> APLVHHHHHHALDENLYFQGALAKYAPDENCPDQNPRLRNWDPGQDSAKQVVIKEGDMLRLTSDATVHSIVIQDGGLLVFGDNKDGSRNITLRTHYILIQDGGALHIGAEKCRYKSKATITLYGKSDEGESMPTFGKKFIGVEAGGTLELHGARKASWTLLARTLNSSGLPFGSYTFEKDFSRGLNVRVIDQDTAKILESERFDTHEYRNESRRLQEFLRFQDPGRIVAIAVGDSAAKSLLQGTIQMIQERLGSELIQGLGYRQAWALVGVIDGGSTSCNESVRNYENHSSGGKALAQREFYTVDGQKFSVTAYSEWIEGVSLSGFRVEVVDGVKLNLLDDVSSWKPGDQIVVASTDYSMYQAEEFTLLPCSECSHFQVKVKETPQFLHMGEIIDGVDMRAEVGILTRNIVIQGEVEDSCYAENQCQFFDYDTFGGHIMIMKNFTSVHLSYVELKHMGQQQMGRYPVHFHLCGDVDYKGGYRHATFVDGLSIHHSFSRCITVHGTNGLLIKDTIGFDTLGHCFFLEDGIEQRNTLFHNLGLLTKPGTLLPTDRNNSMCTTMRDKVFGNYIPVPATDCMAVSTFWIAHPNNNLINNAAAGSQDAGIWYLFHKEPTGESSGLQLLAKPELTPLGIFYNNRVHSNFKAGLFIDKGVKTTNSSAADPREYLCLDNSARFRPHQDANPEKPRVAALIDRLIAFKNNDNGAWVRGGDIIVQNSAFADNGIGLTFASDGSFPSDEGSSQEVSESLFVGESRNYGFQGGQNKYVGTGGIDQKPRTLPRNRTFPIRGFQIYDGPIHLTRSTFKKYVPTPDRYSSAIGF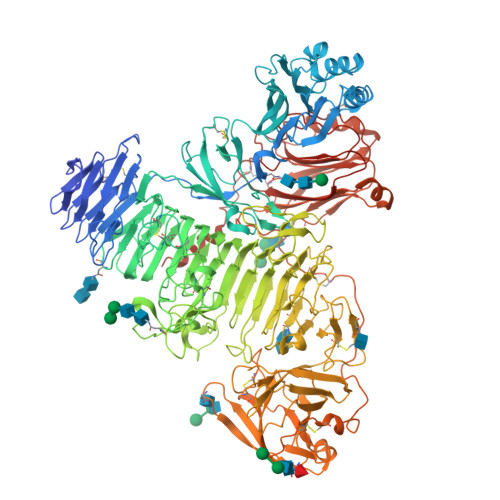LMKNSWQITPRNNISLVKFGPHVSLNVFFGKPGPWFEDCEMDGDKNSIFHDIDGSVTGYKDAYVGRMDNYLIRHPSCVNVSKWNAVICSGTYAQVYVQTWSTQNLSMTITRDEYPSNPMVLRGINQKAAFPQYQPVVMLEKGYTIHWNGPAPRTTFLYLVNFNKNDWIRVGLCYPSNTSFQVTFGYLQRQNGSLSKIEEYEPVHSLEELQRKQSERKFYFDSSTGLLFLYLKAKSHRHGHSYCSSQGCERVKIQAATDSKDISNCMAKAYPQYYRKPSVVKRMPAMLTGLCQGCGTRQVVFTSDPHKSYLPVQFQSPDKAETQRGDPSVISVNGTDFTFRSAGVLLLVVDPCSVPFRLTEKTVFPLADVSRIEEYLKTGIPPRSIVLLSTRGEIKQLNISHLLVPLGLAKPAHLYDKGSTIFLGFSGNFKPSWTKLFTSPAGQGLGVLEQFIPLQLDEYGCPRATTVRRRDLELLKQASKAH> MSTIEHQMHLEKLYNKNQLLPRMRQEFEENSGIDFKAFFAHIGIDYKFGIDAMVQMALHKRADLPTLVGTLRHHCKSAQEVADNLFKMASEDCFNFDPTIDKFIVIYTISDDVQHELDSFQYPLPMVVRPKLLTKNYGTGYFTCNKSVILKKNHTDDDICLDHLNRMNKIPLSINWDVAHMVKNEWANLDKPKEGETRQEFEKRVRAFQKYDRTAHEVMGLLTQEGNKFYLTHRPDKRGRTYSQGYHVNYQGTSWNKAVLEFAEKEVID;> MQTFTAREYLKIDIANNYGLDKEDWDDRIAWFDKNENNLLNLVREAEEPALFYAGVKAWMDVKEGKPIGYPVALDATSSGLQILACLTGDRRAAELCNVVNYRDESGKVKRRDAYTVIYNKMLNTLGKGARIKRNDCKQAIMTALYGSEAKPKEVFGEGIMLNVFESTMNVEAPAVWELNKFWLQCGNPEAFVYHWVMPDGFNVYIKVMVNEVETVH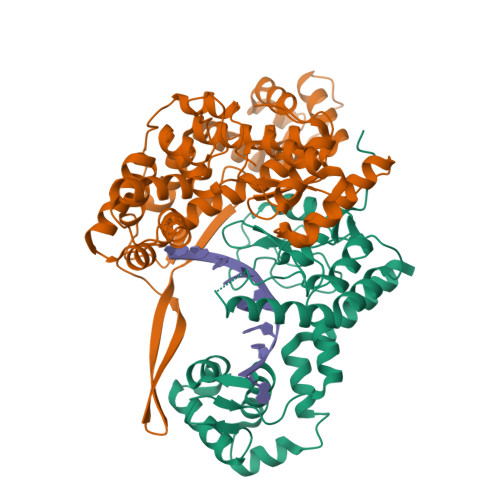FLDKPYDCVRKVQGTEEKTRMLSANTTHSIDGLVVRELVRRCDYDKNQIEYIKALCNGEAEYKASEKNYGKAMELWGYYEKTGFLTARIFDYLDSETIKLVNTQDILDLIESMPKKPFHVLTVHDCFRCLPNYGNDIRRQYNNLLATIAKGDLLSFIMSQVIGQEVTIGKLDPTLWEDVLETEYALS> TIKLIVGLANPGAEYAATRHNAGAWFVDLLAERLRAPLREEAKFFGYTSRVTLGGEDVRLLVPTTFMNLSGKAVAAMASFFRINPDEILVAHDELDLPPGVAKFKLGGGHGGHNGLKDIISKLGNNPNFHRLRIGIGHPGDKNKVVGFVLGKPPVSEQKLIDEAIDEAARCTEMWFTDGLTKA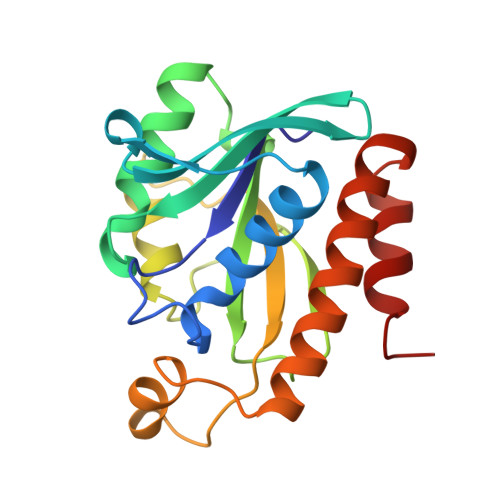TNRLHAFKAQ>MASVKLKGVYKRYPGGVTAVNDFNLDIEDKEFIILVGPSGCGKTTTLRMVAGLEEITEGELYIGDKLVNDVAPKDRDIAMVFQNYALYPHMSVFDNMAFGLKLRKVPKDEIKRRVLEAAKILDIEHLLERKPKALSGGQRQRVALGRAIVRNPKVFLMDEPLSNLDAKLRVQMRTEISKLHQRLQTTFIYVTHDQTEALTMGTRIVVMKDGYIQQVDTPTNLYERPCNMFVAGFIGSPQMNFVNARIEKRGDEMHLLFGKQDIKLPEGK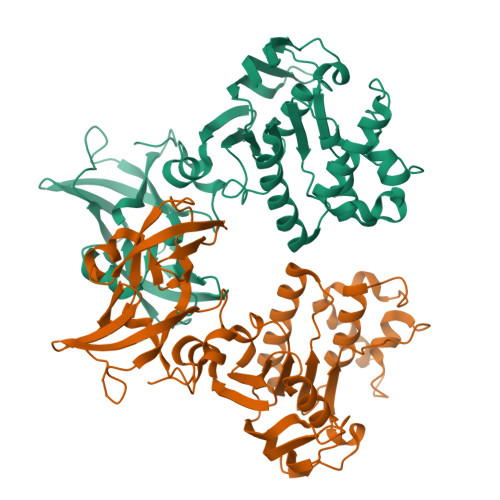AKKLESSEYVGREVVMGIRPENIRDEEIYLESMSENVVEGRVEVVEMLGSETLIYMVIDDFEFTARVNPRSKARPGDVIKVAFDANKIHLFDKETEKTIMN[2x]>VGPKTGEENQVLVPNLNPTPENLEVVGDGFKITSSINLVGEEEADENAVNALREFLTANNIEINSENDPNSTTLIIGEVDDDIPELDEALNGTTAENLKEEGYALVSNDGKIAIEGKDGDGTFYGVQTFKQLVKESNIPEVNITDYPTVSARGIVEGFYGTPWTHQDRLDQIKFYGENKLNTYIYAPKDDPYHREKWREPYPESEMQRMQELINASAENKVDFVFGISPGIDIRFDGDAGEEDFNHLITKAESLYDMGVRSFAIYWDDIQDKSAAKHAQVLNRFNEEFVKAKGDVKPLITVPTEYDTGAMVSNGQPRAYTRIFAETVDPSIEVMWTGPGVVTNEIPLSDAQLISGIYNRNMAVWWNYPVTDYFKGKLALGPMHGLDKGLNQYVDFFTVNPMEHAELSKISIHTAADYSWNMDNYDYDKAWNRAIDMLYGDLAEDMKVFANHSTRMDNKTWAKSGREDAPELRAKMDELWNKLSSKEDASALIEELYGEFARMEEACNNLKANLPEVALEECSRQLDELITLAQGDKASLDMIVAQLNEDTEAYESAKEIAQNKLNTALSSFAVISEKVAQSFIQEALSFDLTL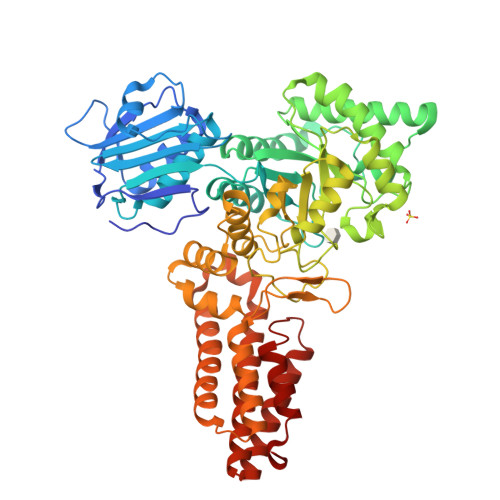I[2x]> MALRAVWLIRHEPGTPLGGTVRFSRRYPTVEKRAKAFNGMTYVPVPEDGPFLRALLFQLRLLDDDKDFMERRDGCSRINKTSIYGLSVGGEELWPVIAFLRDSMIYASVPLVEQALSPRPPLISISGVSQGLELLLGIQDFLYS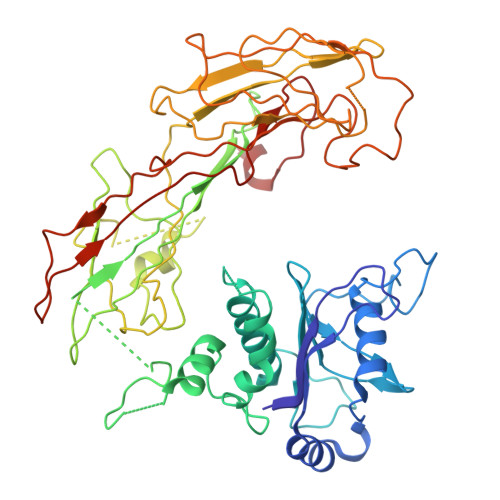SQKNDTDLHTKLSQLPDLLLQACPLGTLLDANLQNSLNSINSVSVTQPQKQPAWKVGAYKGKAQISISITETVKCMQYGKQDIADTWQVAGTVACKCDLEGVMPAVTISLSLPTNGSPLQDIIVHPCVTSLDSAILTSSSIDTMDDSAFSGPYKFPFTPPLESFNLCHYTSQVPVPPILGSYHMKEEGVQLKVTVNFKLHESVRNNFEVCEAHIPFYNRGPITHLEYKASFGQLEVFREKSLLVWIIGQKFPKSMEISLSGTLTFGVKGHNKQPFDHICIGNTAYIKLNFRIADYTLTGCYADQHSVQVFASGKPKISAYRKLISSDYYIWNSKAPAPVTYASLLP> MSRS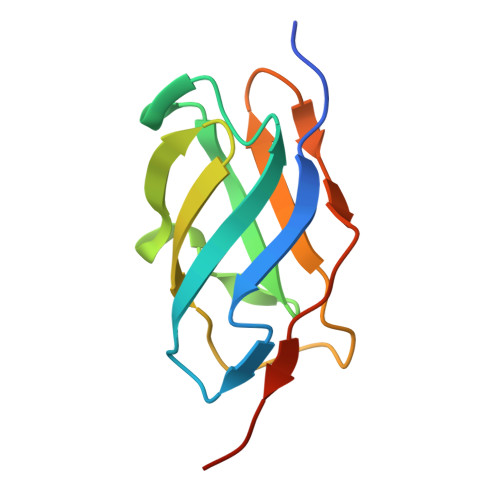RQPPLVTGISPNEGIPWTKVTIRGENLGTGPTDLIGLTICGHNCLLTAEWMSASKIVCRVGQAKNDKGDIIVTTKSGGRGTSTVSFKLLKPEKIG5-S-benzyl-3-({N-[(5-bromo-2-methoxyphenyl)acetyl]-L-valyl}amino)-2,3-dideoxy-5-thio-D-erythro-pentonic acid 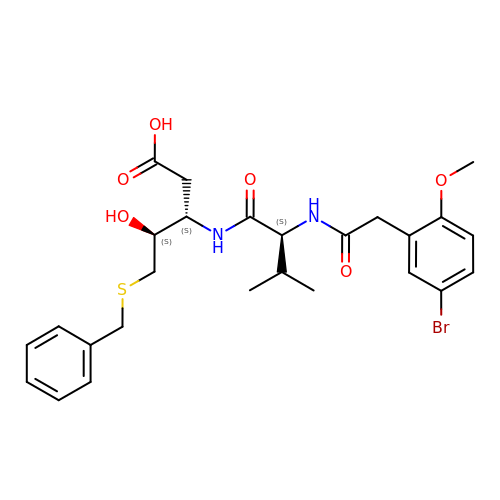| C26 H33 Br N2 O6 S | IQHLJYZLDAEITK-BKSPAHHJSA-N> QWALEDFEIGRPLGKGKFGNVYLAREKQSKFILALKVLFKAQLEKAGVEHQLRREVEIQSHLRHPNILRLYGYFHDATRVYLILEYAPLGTVYRELQKLSKF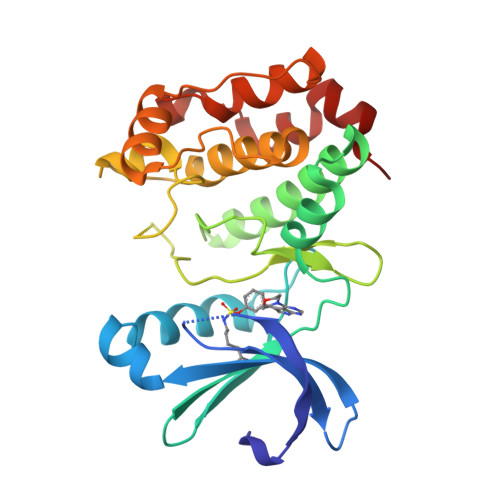DEQRTATYITELANALSYCHSKRVIHRDIKPENLLLGSAGELKIADFGWSVHAPSSRRTTLCGTLDYLPPEMIEGRMHDEKVDLWSLGVLCYEFLVGKPPFEANTYQETYKRISRVEFTFPDFVTEGARDLISRLLKHNPSQRPMLREVLEHPWITANSSK>MANPYERGPNPTDALLEASSGPFSVSEENVSRFGADGFGGGTIYYPRENNTYGAVAISPGYTGTQASVAWLGERIASHGFVVITIDTNTTLDQPDSRARQLNAALDYMINDASSAVRSRIDSSRLAVMG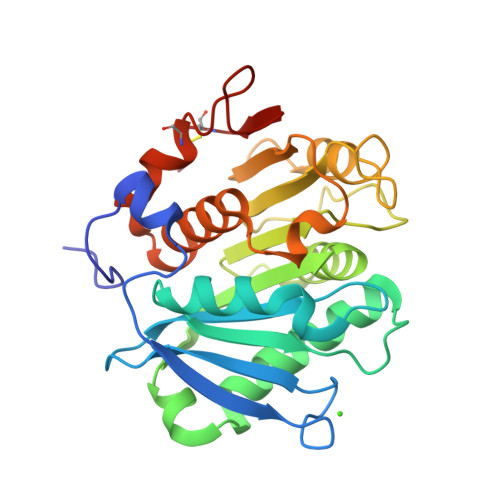HSMGGGGTLRLASQRPDLKAAIPLTPWHLNKNWSSVRVPTLIIGADLDTIAPVLTHARPFYNSLPTSISKAYLELDGATHFAPNIPNKIIGKYSVAWLKRFVDNDTRYTQFLCPGPRDGLFGEVEEYRSTCPFALE[2x]> MKESYYSIGEVSKLANVSIKALRYYDKIDLFKPAYVDPDTSYRYYTDSQLIHLDLIKSLKYIGTPLEEMKKAQDLEMEELFAFYTEQERQIREKLDFLSALE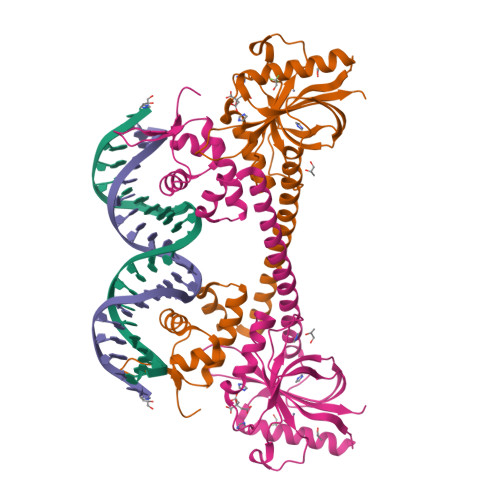QTISLVKKRMKRQMEYPALGEVFVLDEEEIRIIQTEAEGIGPENVLNASYSKLKKFIESADGFTNNSYGATFSFQPYTSIDEMTYRHIFTPVLTNKQISSITPDMEITTIPKGRYACIAYNFSPEHYFLNLQKLIKYIADRQLTVVSDVYQLIIPIHYSPKKQEEYRVEMKIRILDHHHHHH> GSNLAAWKISIPYVDFFEDPSSERKEKKERIPVFCIDVERNDRRAVGHEPEHWSVYRRYLEFYVLESKLTEFHGAFPDAQLPSKRIIGPKNYEFLKSKREEFQEYLQKL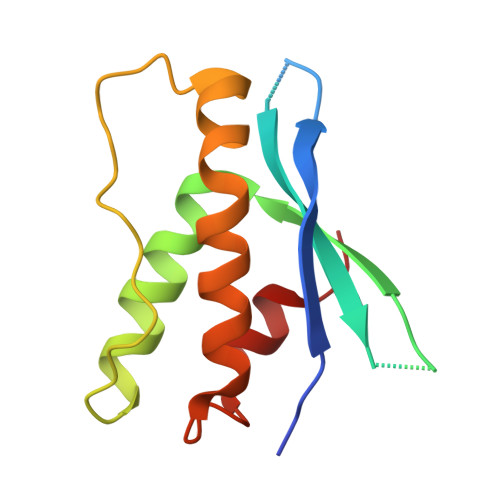LQHPELSNSQLLADFLSPN> SEQTEVLKPRTLADLIRILHQLFAGDEVNVEEVQAIMEAYESDPTEWAMYAKFDQYRYTRNLVDQGNGKFNLMILCWGEGHGSSIHDHTNSHCFLKMLQGNLKETLFAWPDKKSNEMVKKSERVLRENQCAYINDSVGLHRVENISHTEPAVSLHLYS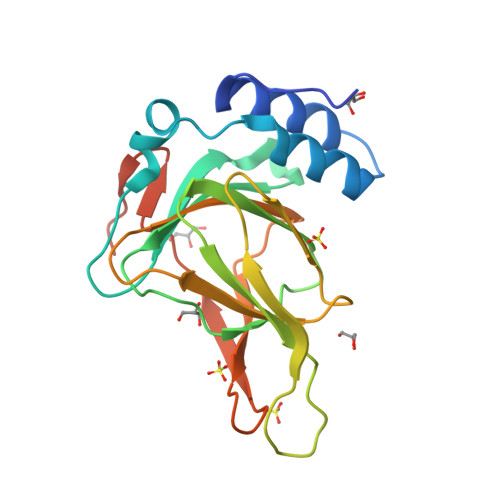PPFDTCHAFDQRTGHKNKVTMTFHSKFGIRTPNATSGSLENN>MKKNGKSQNQPLDFTQYAKNMRKDLSNQDICLEDGALNHSYFLTKKGQYWTPLNQKALQRGIELFGVGNWKEINYDEFSGKANIVELELRTCMILGINDITEYYGKKISEEEQEEIKKSNIAKGKKENKLKDNIYQKLQQMQ[2x];>[2x]DDYLDRLPKSKKGLQGLLQDIEKRILHYKQLFFKEQNEIANGKRSMVPDNSIPICSDVTKLNFQALIDAQMRHAGKMFDVIMMDPPWQLSSSQPSRGVAIAYDSLSDEKIQNMPIQSLQQDGFIFVWAINAKYRVTIKMIENWGYKLVDEITWVKKTVNGKIAKGHGFYLQHAKESCLIGVKGDVDNGRFKKNIASDVIFSERRGQSQKPEEIYQYINQLCPNGNYLEIFARRNNLHDNWVSIGNEL;>[2x]MSLKKGKFQHNQS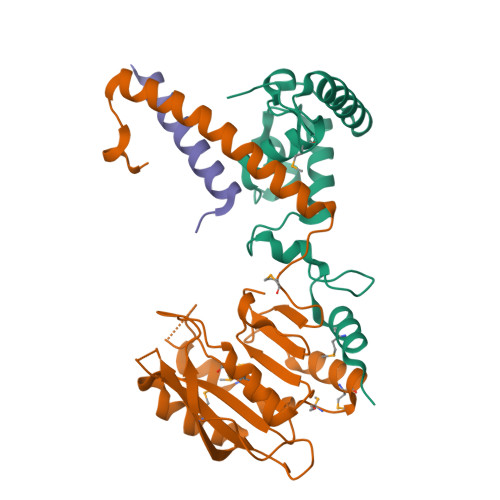KSLWNYTLSPGWREEEVKILKSALQLFGIGKWKKIMESGCLPGKSIGQIYMQTQRLLGQQSLGDFMGLQIDLEAVFNQNMKKQDVLRKNNCIINTGDNPTKEERKRRIEQNRKIYGLSAKQIAEIKLPKVKKHAPQYMTLEDIENEKFTNLEILTHLYNLKAEIVRRLAEQGETIAQPSIIKSLNNLNHNLEQNQNSNSSTETKVTLEQSGKKKYKVLAIEETELQNGPIATNSQKKSINGKRKNNRKINSDSEGNEEDISLEDIDSQESEINSEEIVEDDEEDEQIEEPSKIKKR Nitric oxide (NO) is an important signaling molecule critical in the cardiovascular, neuronal, and immune systems. The enzyme responsible for generating NO is nitric oxide synthase (NOS), a P450-like heme thiolate enzyme that oxidizes l-arginine to NO and L-citrulline. Humans and other mammals express three different NOS isoforms: endothelial NOS (eNOS), neuronal NOS (nNOS), and inducible NOS (iNOS). nNOS is an important therapeutic target since the overproduction of NO by nNOS in the brain is associated with a number of neurodegenerative diseases. Thus, nNOS is an attractive target for therapeutic intervention. In our efforts to develop inhibitors selective for neuronal nitric oxide synthase (nNOS) over endothelial nitric oxide synthase (eNOS), we found that nNOS can undergo conformational changes in response to inhibitor binding that does not readily occur in eNOS. Here, we used a combination of crystallography, mutagenesis, and computational methods to better understand the structural basis for these differences in NOS inhibitor binding.

We first observed protein backbone structural changes with compound 3, followed by observations of the same structural changes in nNOS with many other inhibitors (12 cases in hnNOS and four cases in rnNOS, unpublished results). Compound 4 is a typical example, as shown in Figure 8, where the inhibitor can bind both to the active site and to the BH4 site in hnNOS, triggering backbone changes, but only one inhibitor binds to the active site in heNOS and does not induce backbone changes. However, the crystal structure of heNOS P370N bound with 4 revealed that the inhibitor still binds only at the active site while BH4 is undisturbed, just as in the wild-type heNOS-4 complex. One inhibitor molecule is in the active site, as expected, but the second can displace the BH4 cofactor in nNOS but is much less likely to do so in eNOS. The bulkier His371 in heNOS makes extensive contact with Trp74 and His461 in the neighboring subunit, while Ser607 in hnNOS has no contact at the dimer interface. It appears more likely that the tighter dimer interface in eNOS makes it more difficult to displace BH4 since BH4 sits at the dimer interface and is likely important for stabilizing the dimer.

>[4x]APASLLPPAPEHSPPSSPLTQPPEGPKFPRVKNWEVGSITYDTLSAQAQQDGPCTPRRCLGSLVFPRKLQGRPSPGPPAPEQLLSQARDFINQYYSSIKRSGSQAHEQRLQEVEAEVAATGTYQLRESELVFGAKQAWRNAPRCVGRIQWGKLQVFDARDCRSAQEMFTYICNHIKYATNRGNLRSAITVFPQRCPGRGDFRIWNSQLVRYAGYRQQDGSVRGDPANVEITELCIQHGWTPGNGRFDVLPLLLQAPDEPPELFLLPPELVLEVPLEHPTLEWFAALGLRWYALPAVSNMLLEIGGLEFPAAPFSGWYMSTEIGTRNLCDPHRYNILEDVAVCMDLDTRTTSSLWKDKAAVEINVAVLHSYQLAKVTIVDHHAATASFMKHLENEQKARGGCPADWAWIVPPISGSLTPVFHQEMVNYFLSPAFRYQPDPW>[2x]MQLNNRDLKSIIDNEALAYAMYTVENRAIPNMIDGFKPVQRFVIARALDLARGNKDKFHKLASIAGGVADLGYHHGENSAQDAGALMANTWNNNFPLLDGQGNFGSRTVQKAAASRYIFARVSKNFYNVYKDTEYAPVHQDKEHIPPAFYLPIIPTVLLNGVSGIATGYATYILPHSVSSVKKAVLQALQGKKVTKPKVEFPEFRGEVVEIDGQYEIRGTYKFTSRTQMHITEIPYKYDRETYVSKILDPLENKGFITWDDACGEHGFGFKVKFRKEYSLSDNEEERHAKIMKDFGLIERRSQNITVINEKGKLQVYDNVVDLIKDFVEVRKTYVQKRIDNKIKETESAFRLAFAKAHFIKKVISGEIVVQGKTRKELTEELSKIDMYSSYVDKLVGMNIFHMTSDEAKKLAEEAKAKKEENEYWKTTDVVTEYTKDLEEIK;>MIKNEIKILSDIEHIKKRSGMYIGSSANETHERFMFGKWESVQYVPGLVKLIDEIIDNSVDEGIRTKFKFANKINVTIKNNQVTVEDNGRGIPQAMVKTPTGEEIPGPVAAWTIPKAGGNFGDDKERVTGGMNGVGSSLTNIFSVMFVGETGDGQNNIVVRCSNGMENKSWEDIPGKWKGTRVTFIPDFMSFETNELSQVYLDITLDRLQTLAVVYPDIQFTFNGKKVQGNFKKYARQYDEHAIVQEQENCSIAVGRSPDGFRQLTYVN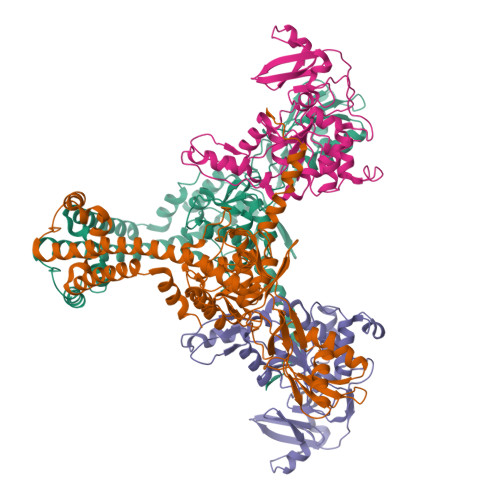NIHTKNGGHHIDCAMDDICEDLIPQIKRKFKIDVTKARVKECLTIVMFVRDMKNMRLIRQTKERLTSPFGEIRSHIQLDAKKISRDILNNEAILMPIIEAALARKLAAEKAAETKAAKKASKAKVHKHIKANLCGKDADTTLFLTEGDSAIGYLIDVRDKELHGGYPLRGKVLNSWGMSYADMLKNKELFDICAITGLVLGEKAFEEKEDGEWFTFELNGDTIIVNENDEVQINGKWITVGELRKNLMKFVKIDSSSVDMKKYKLQNNVRRSIKSSSMNYANVAIMTDADHDGLGSIYPSLLGFFSNWPELFEQGRIRFVKTPVIIAQVGKKQEWFYTVAEYESAKDALPKHSIRYIKGLGSLEKSEYREMIQNPVYDVVKLPENWKELFEMLMGDNADLRKEWMSQHHHHHH[2x]>MRGETLKLKKDKRREAIRQQIDSNPFITDHELSDLFQVSIQTIRLDRTYLNIPELRKRIKLVAEKNYDQISSIEEQEFIGDLIQVNPNVKAQSILDITSDSVFHKTGIARGHVLFAQANSLCVALIKQPTVLTHESSIQFIEKVKLNDTVRAEARVVNQTAKHYYVEVKSYVKHTLVFKGNFKMFYDKRG[2x]

In order to shed light on this fundamental mechanism, we studied S. aureus FapR (SaFapR) a transcription factor that senses the levels of malonyl-CoA, a key intermediate in fatty acid biosynthesis, and modulates the expression of genes involved in fatty acid and phospholipid biosynthesis. FapR has been shown to globally repress the expression of the genes from the fap regulon encoding the soluble FASII system as well as two key enzymes that interface this pathway with the synthesis of phospholipid molecules. Like most transcriptional regulators in bacteria, FapR is a homodimeric repressor. Each protomer consists of a N-terminal DNA-binding domain (DBD) harboring a classical helix-turn-helix motif connected through a linker α-helix (αL) to a C-terminal effector-binding domain (EBD).

The crystal structure of full-length SaFapR in complex with malonyl-CoA, determined at 1.9 Å resolution, revealed a different, more compact conformation of the repressor. Most notably, the two amphipatic linker helices αL, instead of interacting with each other as in the DNA-bound repressor, now bind to either side of the central dimeric EBD. This results in a protein conformation with the two helix-turn-helix domains far apart from each other, corresponding to an incompetent DNA-binding state. The phosphopantetheine and malonyl groups of malonyl-CoA are well defined in the electron density map. The phosphopantetheine group binds within a tunnel at the interface between the two protomers in the SaFapR homodimer, and adopts the same conformation as observed in many acyl-CoA-binding proteins displaying the hot-dog fold. This binding mode results in the complete occlusion of the ligand malonate from the bulk solvent. The charged carboxylate group of malonate is neutralized through a salt bridge with the guanidinium side-chain of Arg110, and makes additional hydrogen bonding interactions with the main-chain nitrogen from Gly111 and the side-chain of Asn119′ from the second protomer. The engagement of Arg110 in malonyl-CoA-binding triggers a local reorganization of hydrogen-bonding interactions and surface reshaping that further stabilize the loop connecting αL to the first β-strand of the hot-dog fold in the non-productive conformation, thus preventing DNA binding. On the other hand, the adenosine 3′-phosphate moiety of malonyl-CoA is largely exposed to the solvent (it is partially disordered in one of the two protomers) and makes no specific contacts with the protein. This implies that SaFapR specifically recognizes the malonyl-phosphopantetheine moiety of the ligand, in agreement with the observation that either malonyl-CoA or malonyl-acyl carrier protein (malonyl-ACP) can indistinctly function as effector molecules.> E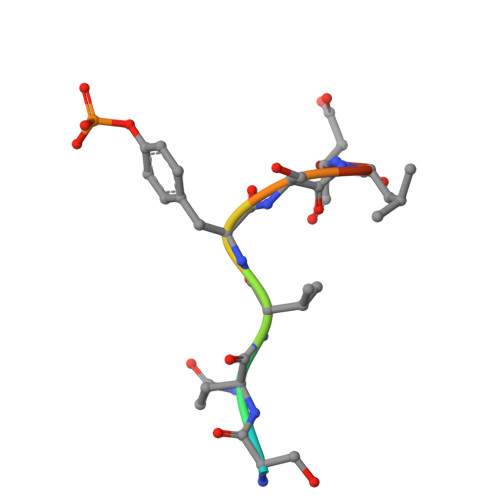SQVYSLDS> MNGIHDTGGAHGYGPVYREPNEPVFRYDWEKTVMSLLPALLANGNFNLDEFRHSIQRMGPAHYLEGTYYEHWLHVFENLLVEKGVLTATEVATGKAASGKTATPVLTPAIVDGLLSTGASAAREEGARARFAVGDKVRVLNKNPVGHTRMPRYTRGKVGTVVIDHGVFVTPDTAAHGKGEHPQHVYTVSFTSVELWGQDASSPKDT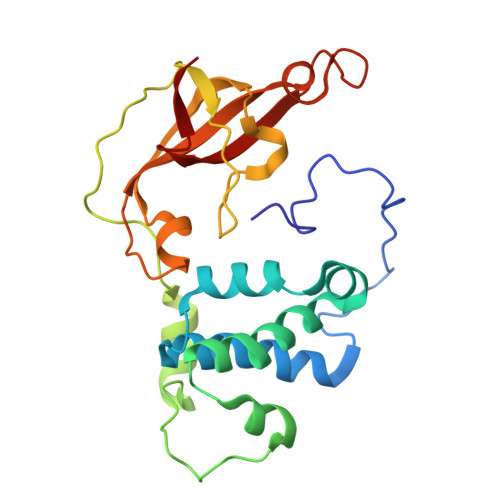IRVDLWDDYLEPA>[2x]G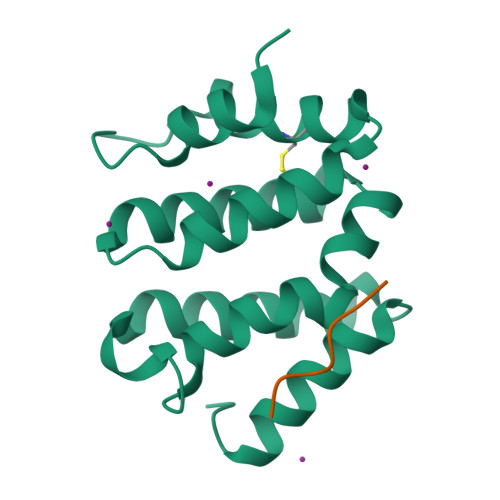SMEPAMEPETLEARINRATNPLNKELDWASINGFCEQLNEDFEGPPLATRLLAHKIQSPQEWEAIQALTVLETCMKSCGKRFHDEVGKFRFLNELIKVVSPKYLGSRTSEKVKNKILELLYSWTVGLPEEVKIAEAYQMLKKQGIVKS;>[2x]SGYHDDSDEDLLE> HNYSEAEIKVREATSNDPWGPSSSLMSEIADLTYNVVAFSEIMSM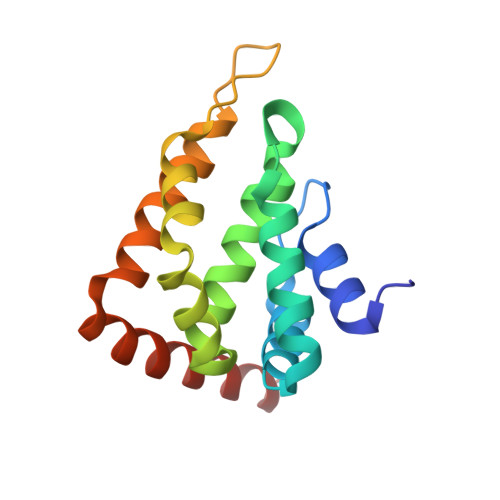IWKRLNDHGKNWRHVYKAMTLMEYLIKTGSERVSQQCKENMYAVQTLKDFQYVDRDGKDQGVNVREKAKQLVALLRDEDRLREERAHALKTKEKLAQTA> MTTTMKISIEFLEPFRMTKWQESTRRNKNNKEFVRGQAFARWHRNKKDNTKGRPYITGTLLRSAVIRSAENLLTLSDGKISEKTCCPGKFDTEDKDRLLQLRQRSTLRWTDKNPCPDNAETYCPFCELLGRSGNDGKKAEKKDWRFRIHFGNLSLPGKPDFDGPKAIGSQRVLNRVDFKSGKAHDFFKAYEVDHTRFPRFEGEITIDNKVSAEARKLLCDSLKFTDRLCGALCVIRFDEYTPAADSGKQTENVQAEPNANLAEKTAEQIISILDDNKKTEYTRLLADAIRSLRRSSKLVAGLPKDHDGKDDHYLWDIGKKKKDENSVTIRQILTTSADTKELKNAGKWREFCEKLGEALYLKSKDMSGGLKITRRILGDAEFHGKPDRLEKSRSVSIGSVLKETVVCGELVAKTPFFFGAIDEDAKQTALQVLLTPDNKYRLPRSAVRGILRRDLQTYFDSPCNAELGGRPCMCKTCRIMRGITVMDARSEYNAPPEIRHRTRINPFTGTVAEGALFNMEVAPEGIVFPFQLRYRGSEDGLPDALKTVLKWWAEGQAFMSGAASTGKGRFRMENAKYETLDLSDENQRNDYLKNWGWRDEKGLEELKKRLNSGLPEPGNYRDPKWHEINVSIEMASPFINGDPIRAAVDKRGTAVVTFVKYKAEGEEAKPVCAYKAESFRGVIRSAVARIHMEDGVPLTELTHSDCECLLCQIFGSEYEAGKIRFEDLVFESDPEPVTFDHVAIDRFTGGAADKKKFDDSPLPGSPARPLMLKGSFWIRRDVLEDEEYCKALGKALADVNNGLYPLGGKSAIGYGQVKSLGIKGDDKRISRLMNPAFDETDVAVPEKPKTDAEVRIEAEKVYYPHYFVEPHKKVEREEKPCGHQKFHEGRLTGKIRCKLITKTPLIVPDTSNDDFFRPADKEARKEKDEYHKSYAFFRLHKQIMIPGSELRGMVSSVYETVTN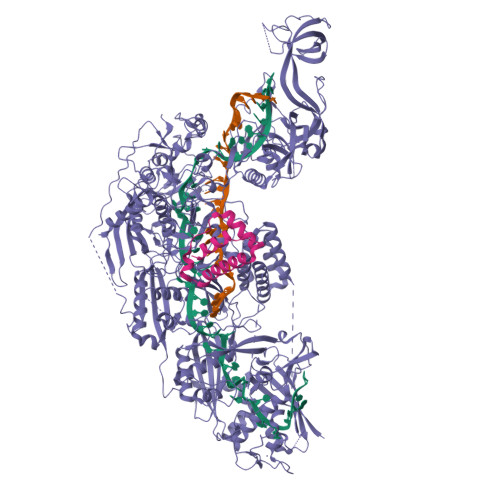SCFRIFDETKRLSWRMDADHQNVLQDFLPGRVTADGKHIQKFSETARVPFYDKTQKHFDILDEQEIAGEKPVRMWVKRFIKRLSLVDPAKHPQKKQDNKWKRRKEGIATFIEQKNGSYYFNVVTNNGCTSFHLWHKPDNFDQEKLEGIQNGEKLDCWVRDSRYQKAFQEIPENDPDGWECKEGYLHVVGPSKVEFSDKKGDVINNFQGTLPSVPNDWKTIRTNDFKNRKRKNEPVFCCEDDKGNYYTMAKYCETFFFDLKENEEYEIPEKARIKYKELLRVYNNNPQAVPESVFQSRVARENVEKLKSGDLVYFKHNEKYVEDIVPVRISRTVDDRMIGKRMSADLRPCHGDWVEDGDLSALNAYPEKRLLLRHPKGLCPACRLFGTGSYKGRVRFGFASLENDPEWLIPGKNPGDPFHGGPVMLSLLERPRPTWSIPGSDNKFKVPGRKFYVHHHAWKTIKDGNHPTTGKAIEQSPNNRTVEALAGGNSFSFEIAFENLKEWELGLLIHSLQLEKGLAHKLGMAKSMGFGSVEIDVESVRLRKDWKQWRNGNSEIPNWLGKGFAKLKEWFRDELDFIENLKKLLWFPEGDQAPRVCYPMLRKKDDPNGNSGYEELKDGEFKKEDRQKKLTTPWTPWASSGLVPRGSHHHHHHH;> MSNPIRDIQDRLKTAKFDNKDDMMNLASSLYKYEKQLMDSSEATLCQQGLSNRPNSFSQLSQFRDSDIQSKAGGQTGKFWQNEYEACKNFQTHKERRETLEQIIRFLQNGAEEKDADDLLLKTLARAYFHRGLLYRPKGFSVPARKVEAMKKAIAYCEIILDKNEEESEALRIWLYAAMELRRCGEEYPENFAEKLFYLANDGFISELYDIRLFLEYTEREEDNNFLDMILQENQDRERLFELCLYKARACFHLNQLNDVRIYGESAIDNAPGAFADPFWDELVEFIRMLRNKKSELWKEIAIKAWDKCREKEMKVGNNIYLSWYWARQRELYDLAFMAQDGIEKKTRIADSLKSRTTLRIQELNELRKDAHRKQNRRLEDKLDRIIEQENEARDGAYLRRNPPCFTGGKREEIPFARLPQNWIAVHFYLNELESHEGGKGGHALIYDPQKAEKDQWQDKSFDYKELHRKFLEWQENYILNEEGSADFLVTLCREIEKAMPFLFKSEVIPEDRPVLWIPHGFLHRLPLHAAMKSGNNSNIEIFWERHASRYLPAWHLFDPAPYSREESSTLLKNFEEYDFQNLENGEIEVYAPSSPKKVKEAIRENPAILLLLCHGEADMTNPFRSCLKLKNKDMTIFDLLTVEDVRLSGSRILLGACESDMVPPLEFSVDEHLSVSGAFLSHKAGEIVAGLWTVDSEKVDECYSYLVEEKDFLRNLQEWQMAETENFRSENDSSLFYKIAPFRIIGFPAE> GSHMSGKARLHYPVTRQGEQVDHYFGQAVADPYRWLEDDRSPETEAWVKAQNAVTQDYLA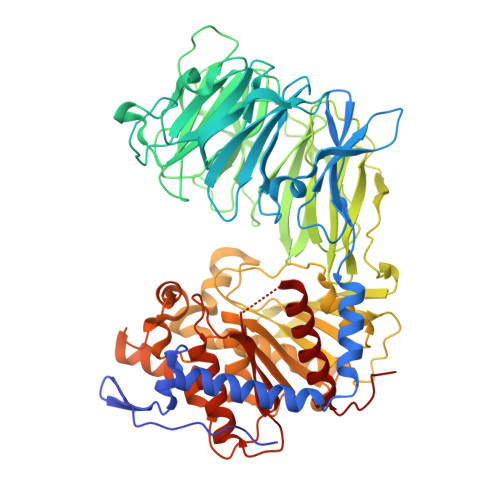QIPYRAAIKEKLAASWNYAKEGAPFREGRYHYFFKNDGLQNQNVLWRQQEGKPAEVFLDPNTLSPDGTTALDQLSFSRDGRILAYSLSLAGSDWREIHLMDVESKQPLETPLKDVKFSGISWLGNEGFFYSSYDKPDGSELSARTDQHKVYFHRLGTAQEDDRLVFGAIPAQHHRYVGATVTEDDRFLLISAANSTSGNRLYVKDLSQENAPLLTVQGDLDADVSLVDNKGSTLYLLTNRDAPNRRLVTVDAANPGPAHWRDLIPERQQVLTVHSGSGYLFAEYMVDATARVEQFDYEGKRVREVALPGLGSVSGFNGKHDDPALYFGFENYAQPPTLYRFEPKSGAISLYRASAAPFKPEDYVSEQRFYQSKDGTRVPLIISYRKGLKLDGSNPTILYGYGGFDVSLTPSFSVSVANWLDLGGVYAVANLRGGGEYGQAWHLAGTQQNKQNVFDDFIAAAEYLKAEGYTRTDRLAIRGGSNGGLLVGAVMTQRPDLMRVALPAVGVLDMLRYHTFTAGTGWAYDYGTSADSEAMFDYLKGYSPLHNVRPGVSYPSTMVTTADHNDRVVPAHSFKFAATLQADNAGPHPQLIRIETNAGHGAGTPVAKLIEQSADIYAFTLYEMGYRELPRQP>GPGSEFRRRRRCQVAFSYLPQNDDELELKVGDIIEVVGEVEEGWWEGVLNGKTGMFPSNFIKELSG[2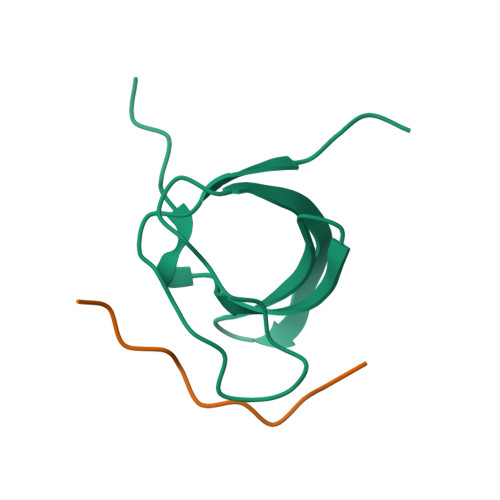x];>RPVPMKRHIFR[2x]>[2x]MTTGLSTAGAQDIGRSSVRPYLEECTRRFQEMFDRHVVTRPTKVELTDAELREVID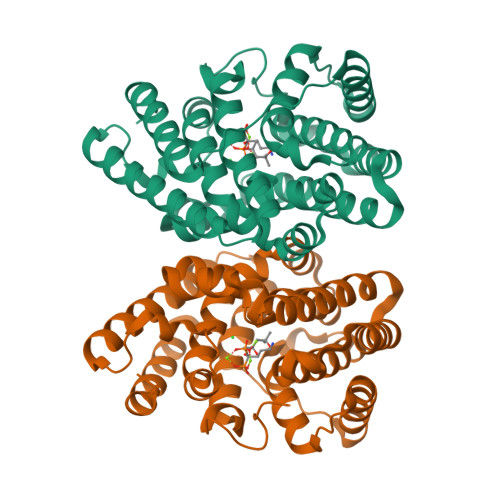DCNAAVAPLGKTVSDERWISYVGVVLWSQSPRHIKDMEAFKAVCVLNCVTFVWDDMDPALHDFGLFLPQLRKICEKYYGPEDAEVAYEAARAFVTSDHMFRDSPIKAALCTTSPEQYFRFRVTDIGVDFWMKMSYPIYRHPEFTEHAKTSLAARMTTRGLTIVNDFYSYDREVSLGQITNCFRLCDVSDETAFKEFFQARLDDMIEDIECIKAFDQLTQDVFLDLIYGNFVGTTSNKRYKTAVNDVNSRIQAAALEHHHHHH>DERRELEKVAVKAIMAAMLGNTDEVREQLQRALEIARESGTLLAVVLALEVVARVAIEAARKGNTDAVREALEVALEIARESGTKVAVVLALEVVARVAIEAARRGNVLAVILALEVALE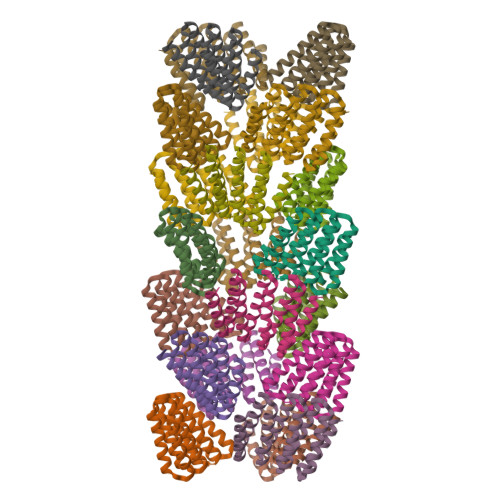IARESGTEEAALLAVEVVVRVSDEAKKQGNAVAVAVAEQVAKKILEES[21x]> MISNDIAIDLGTANTLIYQKGKGIVLNEPSVVALRNVGGRKVVHAVGIEAKQMLGRTPGHMEAIRPMRDGVIADFEVAEEMIKYFIRKVHNRKGFVNPKVIVCVPSGATAVERRAINDSCLNAGARRVGLIDEPMAAAIGAGLPIHEPTGSMVVDIGGGTTEVAVLSLSGIVYSRSVRVGGDKMDEAIISYMRRHHNLLIGETTAERIKKEIGTARAPADGEGLSIDVKGRDLMQGVPREVRISEKQAADALAEPVGQIVEAVKVALEATPPELASDIADKGIMLTGGGALLRGLDAEIRDHTGLPVTVADDPLSCVALGCGKVLEHPKWMKGVLESTLAGSHHHHHH

In non-spherical bacteria, the actin homologue MreB is essential for shape maintenance as depletion of MreB through genetic knockouts or MreB-targeted drug treatment results in misshapen cells that eventually lyse. The MreB fibres are attached to the cell membrane via a hydrophobic loop in Thermotoga maritima as well as Gram+ bacteria and via an additional N-terminal amphipathic helix in Gram− bacteria. Here, we demonstrate that MreB from Caulobacter crescentus forms pairs of antiparallel protofilaments as revealed by crystal structures, an architecture unprecedented among actin-like proteins. The crystal structure of Caulobacter MreB (ΔCcMreBdh) reveals the typical actin fold, containing two domains on either side of a nucleotide binding cleft (Kabsch and Holmes, 1995).

Deleting the N-terminal amphipathic helix and mutating the residues in the hydrophobic loop make the protein (ΔCcMreBdh) less prone to aggregation. In contrast, the crystals of Caulobacter MreB contain doublets that, remarkably, crystallised in an antiparallel arrangement. Although the resolution is low, the entire double protofilament structure of ΔCcMreBdh fits nicely into the 2D averaged EM images with a longitudinal subunit repeat of 5.1 nm and the widths of the doublet encompassing 6.5 nm. (C) Scaled double protofilament from the ΔCcMreBh crystal structure (d_e) was positioned into the EM density obtained from the 2D averaging. Once MreB is in the polymeric state, the presence or absence of nucleotide has very little effect on the overall structure, which is presumably stabilised by inter- and intra-protofilament contacts. The antiparallel arrangement of protofilaments of C. crescentus MreB as revealed by the crystal structure and by EM is unprecedented within the actin family of proteins. It ensures that the amphipathic helix of both protofilaments can bind to the membrane and that both protofilaments are able to interact with bitopic proteins, such as RodZ.>MSAKVYFHETFENRDKWIDSTSSGKALGPFKIVSGKWYGDANNKGLQTSEDNKFYIAAAKLDEEFSNKDKNLIVQYNLKFEQGIDCGGGYIKLLPKKSIESEEKFTPESEYNIMFGPDVCGGSKRTHVIMNYKGKNNLIRKEIKCESDDISHLYTLIIRPNNTYVVKIDGVEKQEGKFDEDWDMLAPKEIDDGSGIANPDYVYDPELYKYDSFAYIGIDVWQVKAGTIYDDILITDDIEEAEKEAKVILERNAAEKKMRDEIKEAEN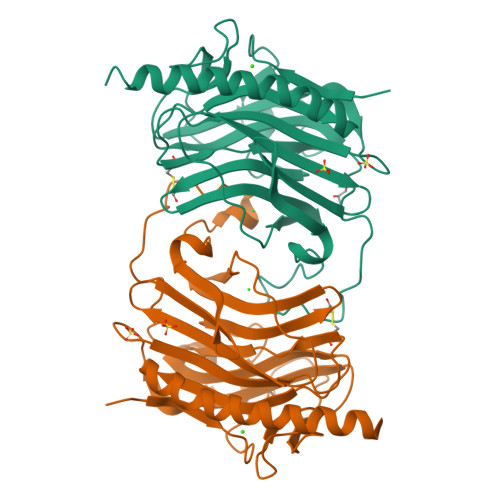GHHHHHH[2x]> IPVIEPLFTKVTEDIPGAEGPVFDKNGDFYIVAPEVEVNGKPAGEILRIDLKTGKKTVICKPEVNGYGGIPAGCQCDRDA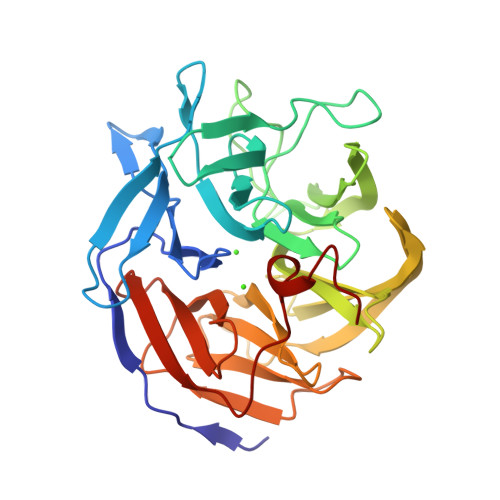NQLFVADMRLGLLVVQTDGTFEEIAKKDSEGRRMQGCNDCAFDYEGNLWITAPAGEVAPADYTRSMQEKFGSIYCFTTDGQMIQVDTAFQFPNGIAVRHMNDGRPYQLIVAETPTKKLWSYDIKGPAKIENKKVWGHIPGTHEGGADGMDFDEDNNLLVANFGSSHIEVFGPDGGQPKMRIRCPFEKPSNLHFKPQTKTIFVTEHENNAVWKFEWQRNGKKQYCETLKFGIF>[2x]MGSHHHHHHGSADITLMNHKYMGNLLH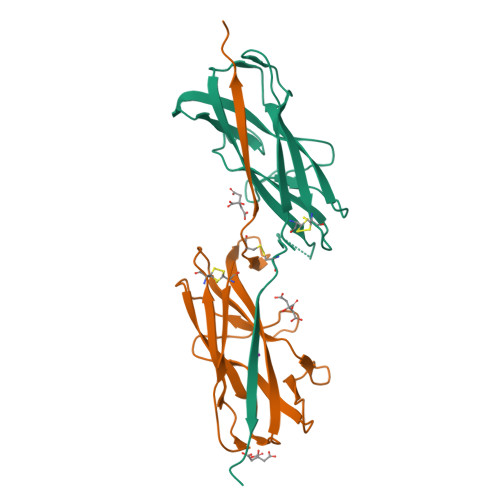DGVKLATGRIICQDTHSGFRVWINARQEGGGAGKYIVQSTEGPQHNLRIRIGGNGWSSFVEKGIQGVFNTIKEDASIFYIEVDGNQQVHPGKYLFSVSGECYIHMDNKQEFIPLCQAATITAQHTVEKLN>[12x]SLKIVVTKFGGSSLADSNQFKKVKGIIDSDANRKYIIPSAPGKRTNKDYKITDLLYLCNAHVKNGIPFDDVFKLIS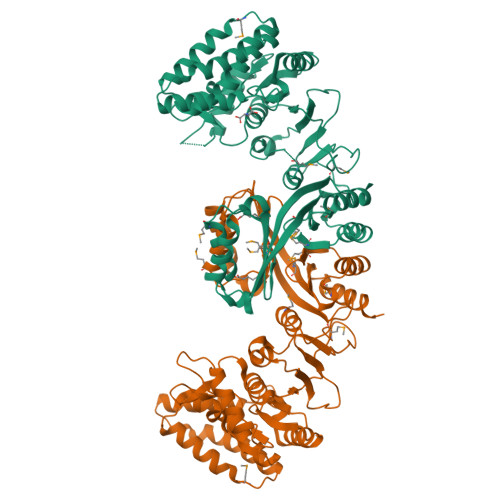QRYTEIVSELNIDMDIAYYLEKVKKNIENGASSDYAASRGEYLNGVILAKYLNAEFIDAAEVIFFDKSGCFDEKKSYEKIKEKVLSCNKAVIPGFYGSSFNGDVKTFSRGGSDVTGSIISAGVNADLYENWTDVSGFLMADPRIVENPKTISKISYKELRELSYMGATVLHEEAIFPVKDSGIPINIKNTNKPSDPGTLILSDTHKEINLGTITGIAGKKNFTVIAIEKALLNSEVGFCRKILSILEMYGVSFEHMPSGVDSVSLVIEDCKLDGKCDKIIEEIKKQCNPDSIEIHPNMALVATVGTGMAKTKGIANKIFTALSKENVNIRMIDQGSSEINVIVGVETVDFEKAVKSIYNAFNEGHHHHHH> GAEIPKERLRAQTNXILLNVLKQGDNYVYGIIKQVKEASNGEMELNEATLYTIFDRLEQDGIISSYWGDESQGGRRKYYRLT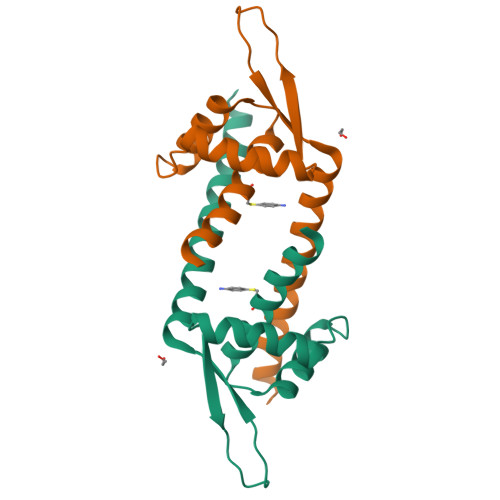EIGHENMRLDIESWSRVDKIIENLEANKKSEAIKSRGGSGG> MGSSHHHHHHSQDPNSMGKLTLLLLAILVWLQYSLWFGKNGIHDYTRVNDDVAAQQATNAKLKARNDQLFAEIDHLNGGQEALEERARNELSMTRPGETFYRLVPDASKRAQSAGQNNR;> MISRVTEALSKVKGSMGSHERHALPGVIGDDL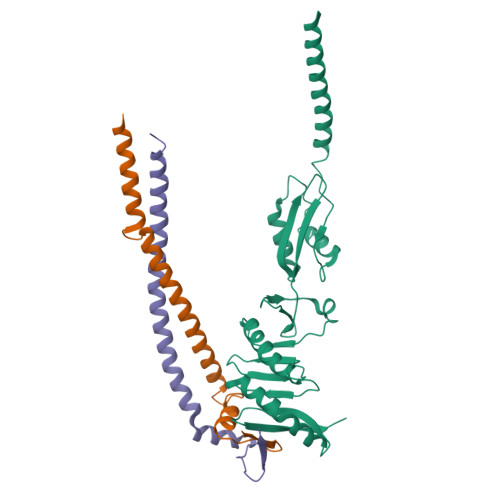LRFGKLPLCLFICIILTAVTVVTTAHHTRLLTAQREQLVLERDALDIEWRNLILEENALGDHSRVERIATEKLQMQHVDPSQENIVVQK;> MSQAALNTRNSEEEVSSRRNNGTRLAGILFLLTVLTTVLVSGWVVLGWMEDAQRLPLSKLVLTGERHYTRNDDIRQSILALGEPGTFMTQDVNIIQTQIEQRLPWIKQVSVRKQWPDELKIHLVEYVPIARWNDQHMVDAEGNTFSVPPERTSKQVLPMLYGPEGSANEVLQGYREMGQMLAKDRFTLKEAAMTARRSWQLTLNNDIKLNLGRGDTMKRLARFVELYPVLQQQAQTDGKRISYVDLRYDSGAAVGWAPLPPEESTQQQNQAQAEQQ(2~{S})-2-azanyl-3-[3-[(2-nitrophenyl)methoxy]-4-oxidanyl-phenyl]propanoic acid | C16 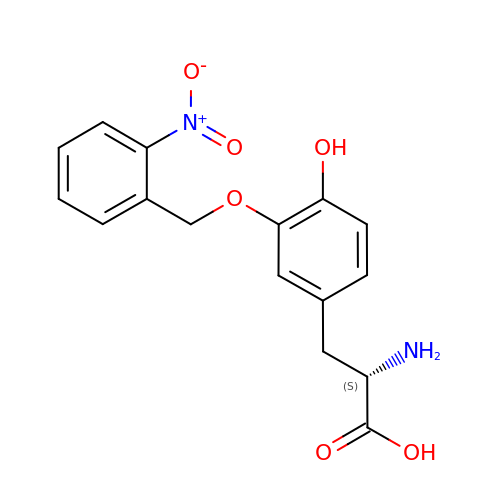H16 N2 O6 | NKOMHGJPHGNQSO-LBPRGKRZSA-N>[2x]MKPVPTYVQDKDESTLMFSVCSLVRDQAKYDRLLESFERFGFTPDKAEFLAADNREGNQFHGFSW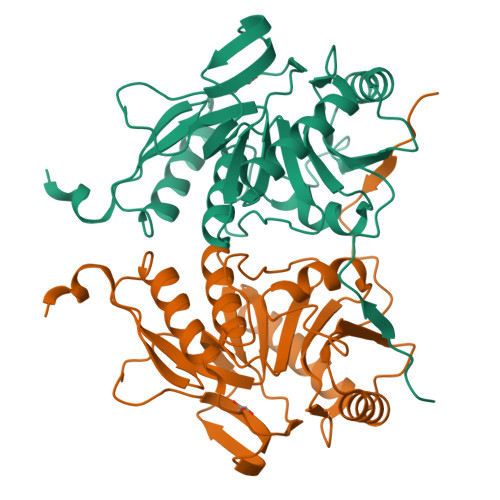HKQMLPRCKGRYVIFCHEDVELVDRGYDDLVAAIEALEEADPKWLVAGVAGSPWRPLNHSVTAQALHISDVFGNDRRRGNVPCRVESLDECFLLMRRLKPVLNSYDMQGFHYYGADLCLQAEFLGGRAYAIDFHLHHYGRAIADENFHRLRQEMAQKYRRWFPGRILHCVTGRVALGGGWYEAR>[2x]KPGAPWWKSAVFYQVYPRSFKDTNGDGIGDFKGLTEKLDYLKGLGIDAIWINPHYASPNTDNGYDISDYREVMKEYGTMEDFDRLMAELKKRGMRLMVDVVINHSSDQHEWFKSSRASKDNPYRDYYFWRDGKDGHEPNNYPSFFGGSAWEKDPVTGQYYLHYFGRQQPDLNWDTPKLREELYAMLRFWLDKGVSGMRFDTVATYSKTPGFPDLTPEQMKNFAEAYTQGPNLHRYLQEMHEKVFDHYDAVTAGQIFGAPLNQVPLFIDSRRKELDMAFTFDLIRYDRALDRWHTIPRTLADFRQTIDKVDAIAGEY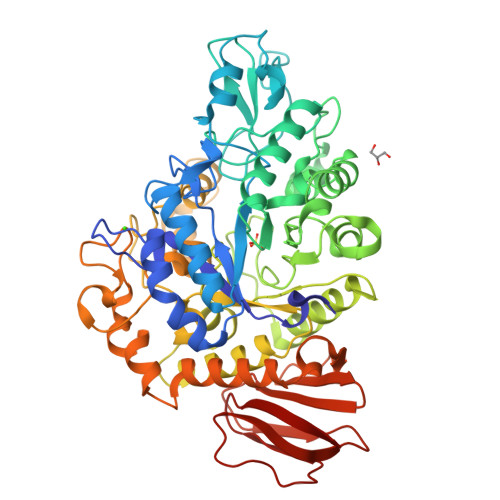GWNTFFLGNHDNPRAVSHFGDDRPQWREASAKALATVTLTQRGTPFIFQGDELGMTNYPFKTLQDFDDIEVKGFFQDYVETGKATAEELLTNVALTSRNNARTPFQWDDSANAGFTTGKPWLKVNPNYTEINAAREIGDPKSVYSFYRNLISIRHETPALSTGSYRDIDPSNADVYAYTRSQDGETYLVVVNFKAEPRSFTLPDGMHIAETLIESSSPAAPAAGAASLELQPWQSGIYKVK~{N}-(2,3-dihydro-1~{H}-inden-2-yl)-3-(piperidin-1-ylcarbonylamino)pyrazine-2-carboxamide | C20 H23 N5 O2 | 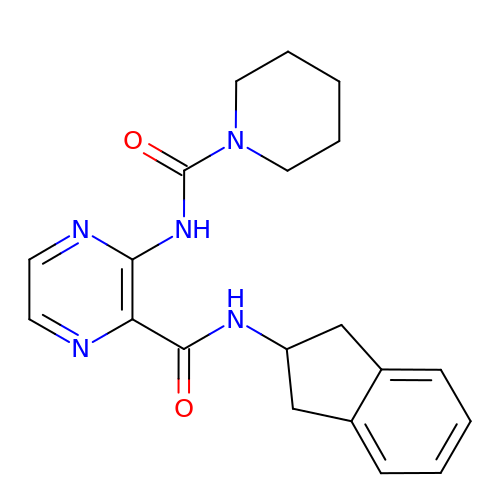AOICKOCLMIPLFS-UHFFFAOYSA-N1-deoxy-1-(8-hydroxy-2,4-dioxo-3,4-dihydropyrimido[4,5-b]quinolin-10(2H)-yl)-D-ribitol 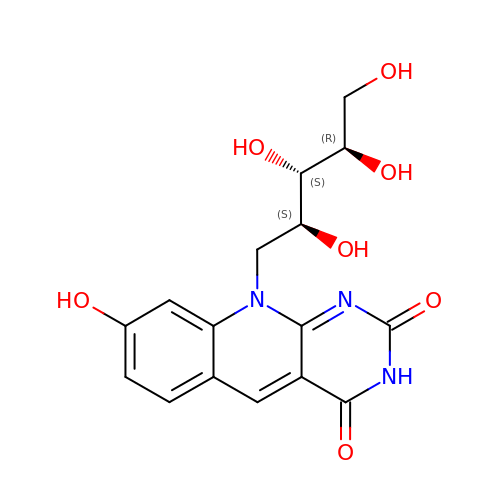| C16 H17 N3 O7 | AUEILLWDYUBWCM-XQQFMLRXSA-N>MSVIHPLQNLLTSRDGSLVFAIIKNCILSFKYQSPNHWEFAGKWSDDFDKIQESRNTTAKEQQGQSSENENENKKLKSNKGDSIKRTAAKVPSPGLGAPPIYSYIRNLRLTSDESRLIACADSDKSLLVFDVDKTSKNVLKLRKRFCFSKRPNAISIAEDDTTVIIA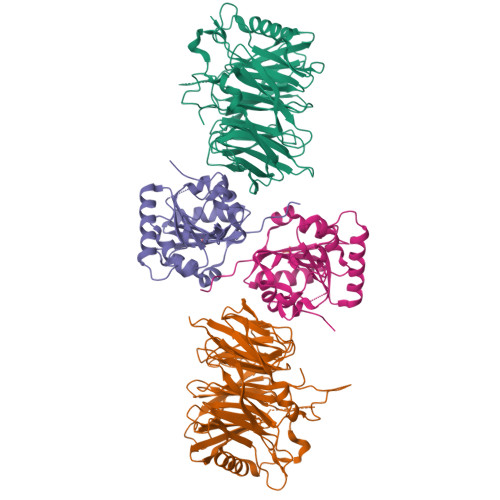DKFGDVYSIDINSIPEEKFTQEPILGHVSMLTDVHLIKDSDGHQFIITSDRDEHIKISHYPQCFIVDKWLFGHKHFVSSICCGKDYLLLSAGGDDKIFAWDWKTGKNLSTFDYNSLIKPYLNDQHLAPPRFQNENNDIIEFAVSKIIKSKNLPFVAFFVEATKCIIILEMSEKQKGDLALKQIITFPYNVISLSAHNDEFQVTLDNKESSGVQKNFAKFIEYNLNENSFVVNNEKSNEFDSAIIQSVQGDSNLVTKKEEIYPLYNVSSLRKHGEHYSHHHHHH[2x];>VQEGQKIDLPKKRYYRQRAHSNPFSDHQLEYPVSPQDMDWSKLYPYYKNAENGQMTKKVTIADIGCGFGGLMIDLSPAFPEDLILGMEIRVQVTNYVEDRIIALRNNTASKHGFQNINVLRGNAMKFLPNFFEKGQLSKMFFCFPDPHFKQRKHKARIITNTLLSEYAYVLKEGGVVYTITDVKDLHEWMVKHLEEHPLFERLSKEWEENDECVKIMRNATEEGKKVERKKGDKFVACFTRLPTPAILHHHHHH[2x]To generalize this engineering approach for crystal contacts, a non-ADH-homologous enzyme was selected to apply the established strategies to the Nostoc sp. PCC 1720 ene reductase (NostocER). This oxidoreductase from the old yellow enzyme family (OYE, EC 1.6.99.1) catalyzes the trans-hydrogenations of activated alkenes, demonstrating its industrial relevance as a biocatalyst. As OYEs are strongly dependent on cost-intensive NADPH as a cofactor, Mähler et al. engineered NADH-accepting variants (NostocER1) by exchanging NostocER loop regions at cofactor-binding sites to ER loop regions from Achromobacter sp. JA81 and Acaryochloris marina with a higher NADH affinity. For this study, the NostocER1 Loop1,5 variant (NostocER1-L1,5) was selected as an example protein for the rational introduction of Lys–Glu interactions at crystal contacts to demonstrate the impact of rational single amino acid exchanges on the crystallizability of proteins and enhance protein crystallization.

Reducing the protein concentration from 10 g L−1 to 5 g L−1 led to a decrease in the crystal amount for all the tested NspER1-L1,5 variants, with D352K being the mutant that formed crystals of the smallest size but in the highest amount. Mutants D352K and T354K crystallizing in the same space group P1211 as the wild type showed, again, an excellent agreement in crystal packing. The crystal contact at position D352K is not conform to expectations and is quite complex, with more than one amino acid residue interacting with D352K within approx. 10 Å. A sodium ion (lilac) also seemed to participate in the interaction complex. Introducing a lysine at any of the neighboring NspER1-L1,5 positions Q350, (D352), and T354 led to an interaction with the intermolecular amino acid residue of E25/27. The neighboring NspER1-L1,5 mutants Q350K, D352K, and T354K led to an interaction with intermolecular E25/27 and an increase in crystallizability (Section 3.2, Section 3.3 and Section 3.4), with the strongest impact for T354K. Validating the molecular structure of the NspER1-L1,5 mutants, for 67% (4/6) of the analyzed crystal structures, the correct intermolecular interaction partner was assumed (except for D352K; and Q263K: E146 instead of E44, data not shown).

>[2x]MGHHHHHHGSGSTNINLFSSYQLGELELPNRIVMAPLTRSRAGEGNVPHQLNAIYYGQRASAGLIIAEATQVTPQGQGYPHTPGIHSPEQVAGWKLVTDTVHQQGGRIFLQLWHVGRISHPDLQPDGGLPVAPSAIAPKGEVLTYEGKKPYVTPRALDTSEIPAIVEQYRQGAANALAAGFDGVEIHAANGYLIDQFLRDGTNQRTDEYGGAIENRARLLLEVTEAITSVWDSQRVGVRLSPLTTLNGCVDSHPLETFGYVAQALNRFNLSYLHIFEAIDADIRHGGTVVPTSHLRDRFTGTLIVNGGYTREKGDTVIANKAADLVAFGTLFISNPDLPERLEVNAPLNQAKPTTFYGGGEKGYTDYPFLAVANK tert-butyl [2-(2-{[(2P)-2-{4-[4-(2-amino-2-oxoethyl)-2-fluoroanilino]thieno[2,3-d]pyridazin-7-yl}phenyl]oxy}ethoxy)ethyl]carbamate | C29 H32 F N5 O5 S | 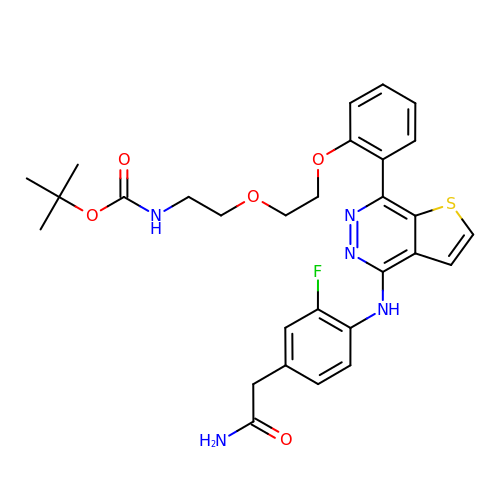NFCHONNVHGPRMI-UHFFFAOYSA-N>[2x]GNNILNSNESRLNVNENNILREKFENYARIVFQFNNSRQANGNFDIANEFISILSSANGTRNAQLLESWKILESMKSKDINIVEVGKQY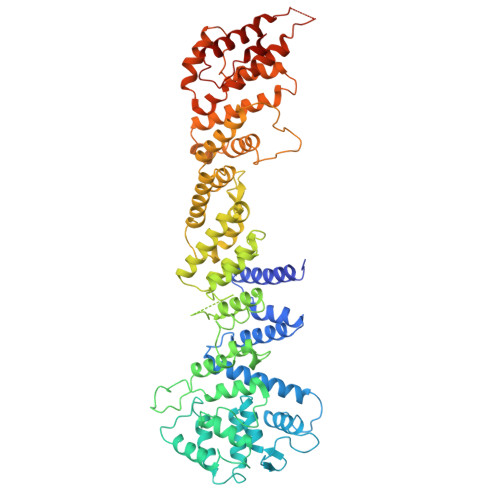LEQQFLQYTDNLYKKNMNEGLATNVNKIKSFIDTKLKKADKSWKISNLTVINGVPIWALIFYLLRAGLIKEALQVLVENKANIKKVEQSFLTYFKAYASSKDHGLPVEYSTKLHTEYNQHIKSSLDGDPYRLAVYKLIGRCDLSRKNIPAVTLSIEDWLWMHLMLIKEKDAENDPVYERYSLEDFQNIIISYGPSRFSNYYLQTLLLSGLYGLAIDYTYTFSEMDAVHLAIGLASLKLFKIDSSTRLTKKPKRDIRFANILANYTKSFRYSDPRVAVEYLVLITLNEGPTDVELCHEALRELVLETKEFTVLLGKIGRDGARIPGVIEERQPLLHVRDEKEFLHTITEQAARRADEDGRIYDSILLYQLAEEYDIVITLVNSLLSDTLSASDLDQPLVGPDDNSETNPVLLARRMASIYFDNAGISRQIHVKNKEICMLLLNISSIRELYFNKQWQETLSQMELLDLLPFSDELSARKKAQDFSNLDDNIVKNIPNLLIITLSCISNMIHILNESKYQSSTKGQQIDSLKNVARQCMIYAGMIQYRMPRETYSTLINIDVSL>GMNYQNDDLRIKEIKELLPPVALLEKFPATENAANTVAHARKAIHKILKGNDDRLLVVIGPCSIHDPVAAKEYATRLLALREELKDELEIVMRVYFEKPRTTVGWKGLINDPHMDNSFQINDGLRIARKLLLDINDSGLPAAGEFLDMITPQYLADLMSWGAIGARTTESQVHRELASGLSCPVGFKNGTDGTIKVAIDAINAAGAPHCFLSVTKWGHSAIVNTSGNGDCHIILRGGKEPNYSAKHVAEVKEGLNKAGLPAQVMIDFSHANSSKQFKKQMDVCADVCQQIAGGEKAI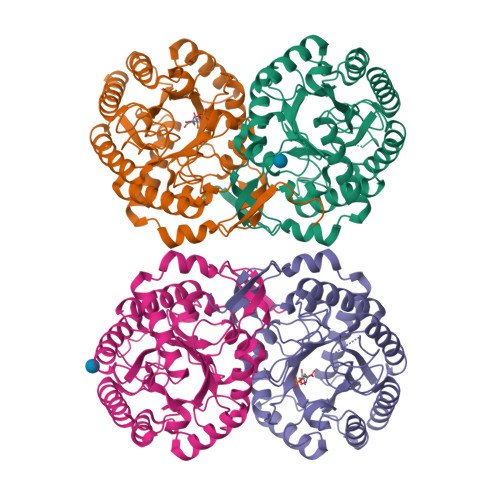IGVMVESHLVEGNQSLESGEPLAYGKSITDACIGWEDTDALLRQLANAVKARRG[4x]> TIDQWLLKNAKEDAIAELKKAGITEPHVISFINHAPYVSHVNGLKNAILKAH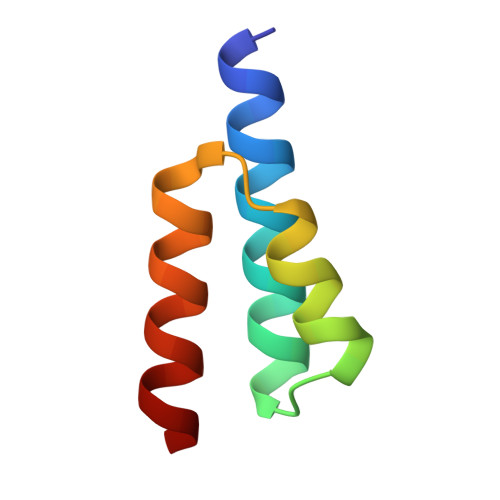A> 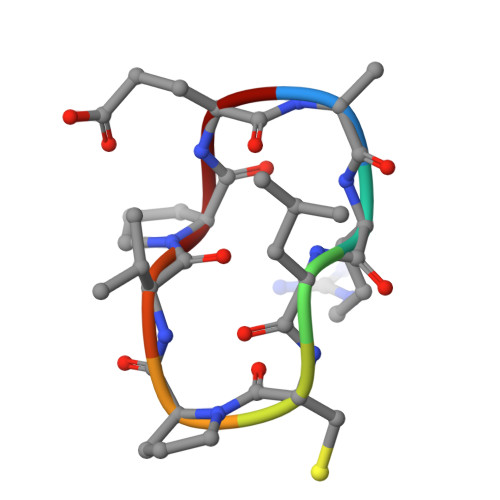RRLCPVPE>[2x]TNVISTLDLNLLTKGGGSWNVDGVNMKKSAVTTFDGKRVVKAVYDKNSGTSANPGVGGFSFSAVPDGLNKNAITFAWEVFYPKGFDFARGGKHGGTFIGHGAASGYQHSKTGASNRIMWQEKGGVIDYIYPPSDLKQKIPGLDPEG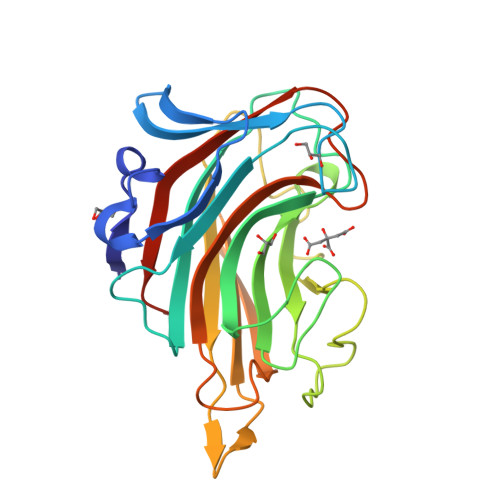HGIGFFQDDFKNALKYDVWNRIEIGTKMNTFKNGIPQLDGESYVIVNGKKEVLKRINWSRSPDLLISRFDWNTFFGGPLPSPKNQVAYFTNFQMKKYELEHHHHHH> GPNMFFMPKRKIPDPIDRLRRANLACEDDKLMIYGLPWMTTQ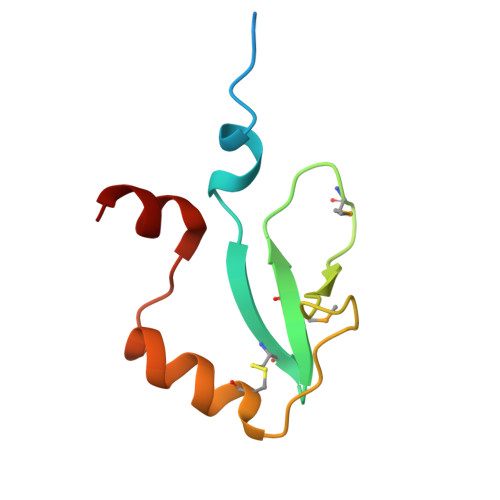TSALSINSKPIVYKDCAKLLRSINGSQPVSLNDVLRR> MYGDLGNKLVLEAKRTKQLYARSNQDVNLPMYHEDIIRNILKEVSNLRKNTEYLKEQQQLGMLDDKVAKCQYFVTL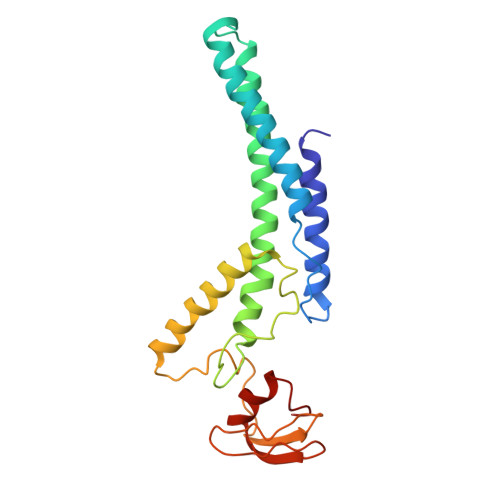LCMERNKRCLLAYQRLRTDILDSMAWNNNGLDLMSSITFSQQDTNNLSHQEQEYLKEYCDLITDLKSGDLVDIDLSGSLVPPSDAFIDVRVLKDAGEIQTEYGVFNLIKDSQFFVQQSDVERLIQQGYLQLI>[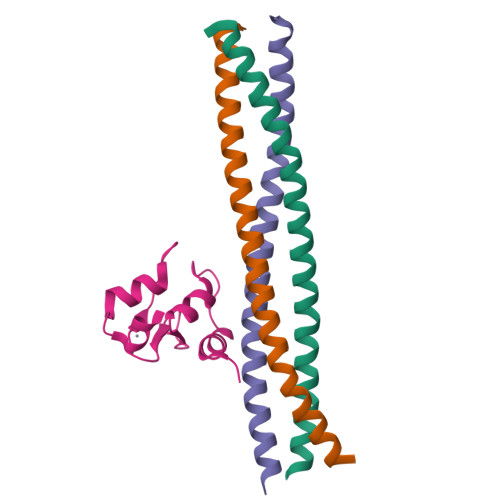2x]SELLQRCESLEKKTATFENIVCVLNREVERVAMTAEACSRQHRLDQDKIEALSSKVQQLERSIGLE;> MFMKEKLLAELEGKLRVFENIVAVLNKEVEASHLALATSIHQSQLDRERILSLEQRVVELQQTLA;> MLSCELYRMSTYSTFPAGVPVSERSLARAGFYYTGVNDKVKCFCCGLMLDNWKRGDSPTEKHKKLYPSCRFVQSL> MMKAKVIDAVSFSYILRTVGDFLSEANFIVTKEGIRVSGIDPSRVVFLDIFLPSSYFEGFEVSQEKEIIGFKLED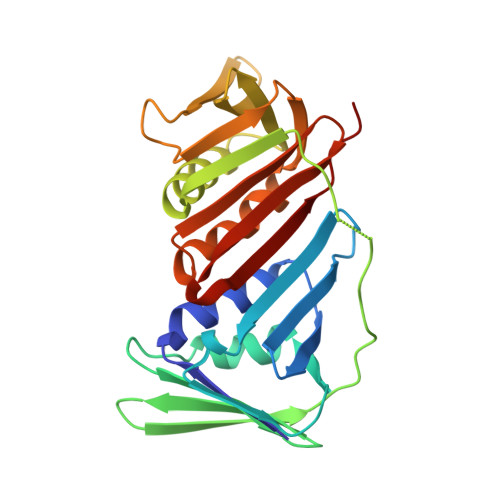VNDILKRVLKDDTLILSSNESKLTLTFDGEFTRSFELPLIQVESTQPPSVNLEFPFKAQLLTITFADIIDELSDLGEVLNIHSKENKLYFEVIGDLSTAKVELSTDNGTLLEASGADVSSSYGMEYVANTTKMRRASDSMELYFGSQIPLKLRFKLPQEGYGDFYIAPRAD> GTLSSEKKAKKVRFYRNGDRYFKGIVYA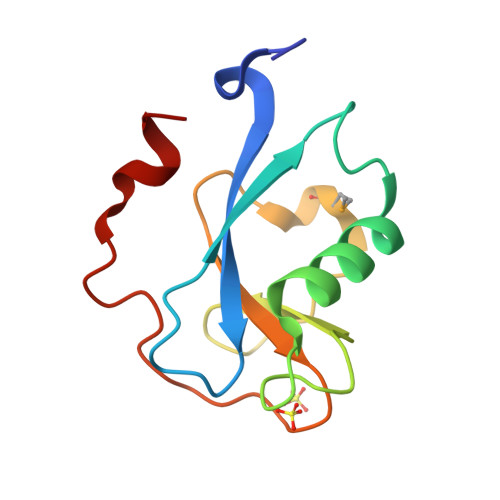ISPDRFRSFEALLADLTRTLSDNVNLPQGVRTIYTIDGLKKISSMDQLVEGESYVCGSIEPFKKLEYTKNVNPNWSVNV> MKTETLYQDPVWFQDLSVIFKRPSEIIPTRDQSDSERINAMVRLVLYCSFAVALIRQNYLYAILGLAIIAIISLAYALGAKKTKSNEAYGNIRPYSVKRSKKSCSKSSANNPFSNATVGALLDNEARPPACSYDDNDMASTMRKNFNKGLFRNLDDVYEVENSQRQFYTMPVTTAAPDLTAFGQFLYGSKGKTCKEDPSACTP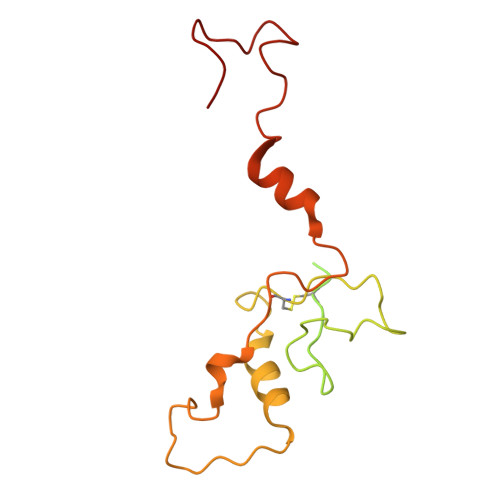AFATRDG(3-EXO)-3-(10,11-DIHYDRO-5H-DIBENZO[A,D][7]ANNULEN-5-YLOXY)-8,8-DIMETHYL-8-AZONIABICYCLO[3.2.1]OCTANE | C24 H30 N O | 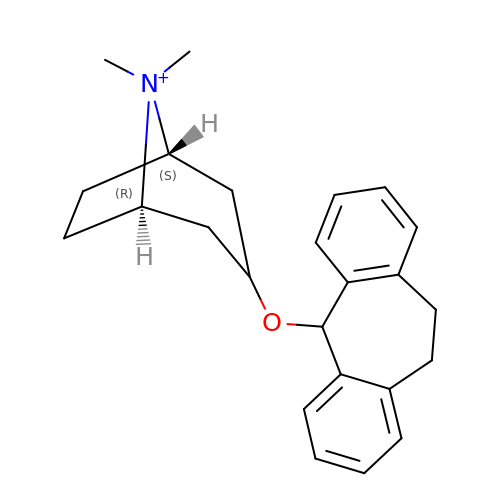BADPXOSJBUEVTR-WKCHPHFGSA-N> MGSDKIHHHHHHMVDTHAHLHFHQFDDDRNAVISS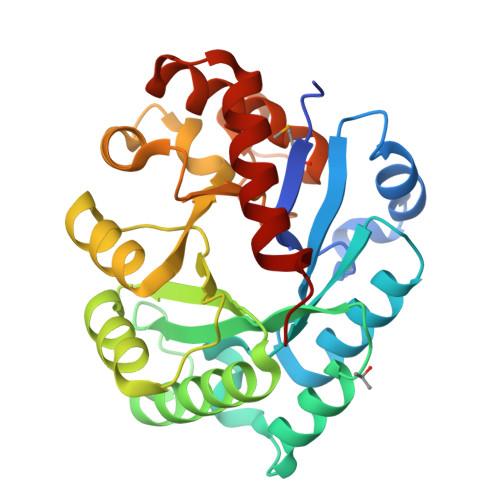FEENNIEFVVNVGVNLEDSKKSLDLSKTSDRIFCSVGVHPHDAKEVPEDFIEHLEKFAKDEKVVAIGETGLDFFRNISPAEVQKRVFVEQIELAGKLNLPLVVHIRDAYSEAYEILRTESLPEKRGVIHAFSSDYEWAKKFIDLGFLLGIGGPVTYPKNEALREVVKRVGLEYIVLETDCPFLPPQPFRGKRNEPKYLKYVVETISQVLGVPEAKVDEATTENARRIFLEVKE> GSPDPRAELDSTVLLTRSLLADTRQLAAQLRDKFPADGDHNLDSLPTLPAIDYALGALQLPGVLTRLRADLLSYLRHVQWLRRAGGSSLKTLEPELGTLQARLDRLLRRLQLLMSRLALPQPPPDPPAPPLAP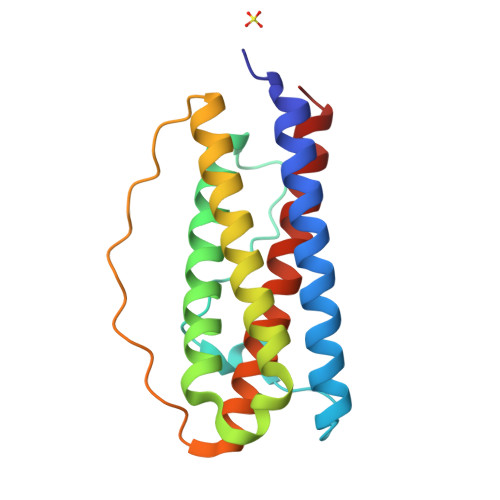PSSAAGGIRAAHAILGGLHLTLDWAVRGLLLLKTRL The role of clathrin is well established in endocytosis, but has also been extended to mitosis, during which clathrin is an essential player of microtubule stability (Royle, 2012; Rondelet et al, 2020). Clathrin classically interacts with its adaptors via clathrin adaptor motifs, such as the LIxF‐motif (Dell'Angelica, 2001; Willox & Royle, 2012; Benz et al, 2022). HURP, in turn, is a microtubules binding protein, the knockdown of which results in a mitotic delay (Wong & Fang, 2006). Among the novel phospho‐modulated interactions, we highlight the interaction between the clathrin N‐terminal domain (NTD) and the mitotic spindle protein Hepatoma‐upregulated protein (HURP).

To shed light on the structural details of the complex, we co‐crystallised a pS839 HURP826–846 peptide with the clathrin NTD. The protein crystallised as a dimer and the peptide bound to the binding pocket 1 in both monomers but was also found to bind to pocket 3 in one of the monomers. In pocket 1, the phosphate group is clamped between the basic residues R64 and K96 (in 4.2 and 2.7 Å distance, respectively) and hence at an appropriate distance to form salt bridges with the phosphate group. In comparison, only one basic residue (K227) was found in vicinity of the phosphate group in pocket 3. Both pockets can hence accommodate the LIxF‐motif, although pocket 1 appears to be the preferred binding pocket due to the observed occupancy and due to a better accommodation of the phosphate group. Superimposition with previously reported structures of the clathrin NTD with a LIxFD‐containing peptide shows that the acidic residue on the bound peptide assumes a similar, but not identical orientation as the phosphorylated serine in pS839 HURP826–846. Further, HURP is highly phosphorylated during mitosis, suggesting that the proline‐directed phosphorylation on S839 is a CDK target (Hsu et al, 2004; Yu et al, 2005; Wong & Fang, 2006), which prompted us to investigate the interaction in this cell cycle stage. We found that phosphorylation of S839 in the HURP832–846 peptide results in a 20‐fold increase in affinity, as demonstrated by both FP and ITC experiments (HURP832–846: FP: KD ≈ 150 μM and ITC: KD ≈ 250 μM, pS839 HURP: FP: KD < 3 μM and ITC KD = 5 μM; Fig 6A and B, Table 1, and Dataset EV10). Nonetheless, overlaying of the crystal structures with complexed HURP or GTSE1 peptides suggests that the two proteins could compete for binding. In conclusion, the association of HURP and clathrin through the C‐terminal LIxF‐motif and enabled by S839 phosphorylation is required for the mitotic function of HURP.

>[2x]MAQILPIRFQEHLQLQNLGINPANIGFSTLTMESDKFICIREKVGEQAQVVIIDMNDPSNPIRRPISADSAIMNPASKVIALKAGKTLQIFNIEMKSKMKAHTMTDDVTFWKWISLNTVALVTDNAVYHWSMEGESQPVKMFDRHSSLAGCQIINYRTDAKQKWLLLTGISAQQNRVVGAMQLYSVDRKVSQPIEGHAASFAQFKMEGNAEESTLFCFAVRGQAGGKLHIIEVGTPPTGNQPFPKKAVDVFFPPEAQNDFPVAMQISEKHDVVFLITKYGYIHLYDLETGTCIYMNRISGETIFVTAPHEATAGIIGVNRKGQVLSVCVEEENIIPYITNVLQNPDLALRMAVRNNLAGAEELF;>YRHISFGGNLITFSPLQPGEF[3x]>[3x]XQARSDIEKLKEAIRDTNKAVQSVQSSIGNLIVAIKSVQDYVNKEIVPSIARX;>[3x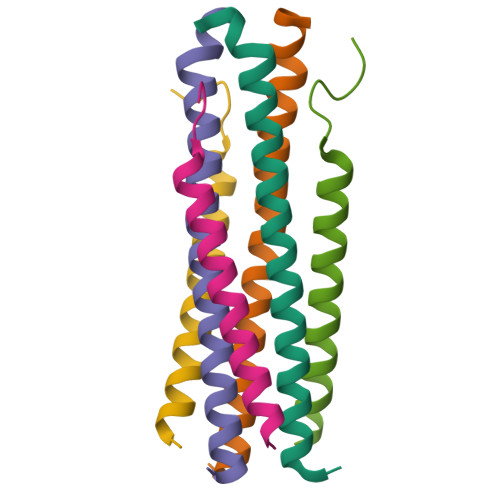]XVALDXIDISIVLNKIKSQLEESKEWIRRSNKILDSIX> IDHWQVDYTHYEDKIILVWVETNSGLIYAERVKGETG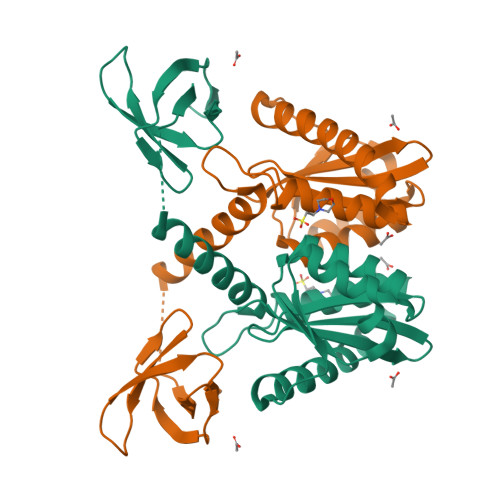QEFRVQTMKWYAMFAPKSLQSDNGPAFVAESTQLLMKYLGIEHTTGIPWNPQSQALVERTHQTLKNTLEKLIPMFNAFESALAGTLITLNIKRKGGLGTSPMDIFIFNKEQQRIQQQSKSKQEKIRFCYYRTRKRGHPGEWQGPTQVLWGGDGAIVVKDRGTDRYLVIANKDVKFIPPPKEIQKE An increasing number of surface‐associated proteins identified in Gram‐positive bacteria are characterized by intramolecular cross‐links in structurally conserved thioester, isopeptide, and ester domains (TIE proteins). TEDs are predicted at the distal end of a large number of surface proteins from Gram‐positive bacteria, and the name TIE (thioester, isopeptide, ester) proteins have been introduced for this family. Internal thioester bonds, formed between Cys and Gln side‐chains and first identified in the second thioester domain (TED) of the Streptococcus pyogenes minor pilin Cpa,3 play a negligible role in protein stability, but are suggested to mediate covalent bacterial adhesion. Structures of Bacillus anthracis, vancomycin‐resistant Staphylococcus aureus, and vancomycin‐resistant Enterococcus faecium TEDs show a head domain with Class I topology extended by a β‐sandwich; the latter contributes the thioester bond‐forming Gln via a β‐hairpin insertion into the head domain.

The B. anthracis BaTIE and the 86 kDa E. faecium EfmTIE86 proteins are predicted to comprise a Class II TED as well as three and five CnaB‐type isopeptide domains (IPDs), respectively. In addition to a TED and four IPDs, the S. aureus SaTIE protein is predicted to also contain two ester domains [Fig. 1(A)]. SaTIE is the only TIE protein so far identified in S. aureus. SaTIE‐TED (Gln254‐Gly502) and EfmTIE86‐TED (Asp39‐Ala314) were determined by ESI‐MS to be 17 Da lighter than predicted (suggesting the presence of a thioester bond), and readily yielded high‐quality crystals. SaTIE‐TED and EfmTIE86‐TED crystal structures were determined using Se‐SAD phasing and standard refinement procedures. Continuous electron density between Cys and Gln side‐chains either previously shown or predicted to form thioesters (SaTIE‐TED: Cys296 + Gln467,5 EfmTIE86‐TED: Cys88 + Gln292) confirmed the presence of these bonds. Despite pairwise identities of 18–23%, all three Class II TEDs in this study display very similar tertiary structures. In Class II TEDs, this loop is extended by approximately 15 residues, and covers the cleft between the β‐barrel and α‐helical subdomains. The specificity loop also contributes to forming a pore over 8 Å deep, the second restriction on access to the thioester bond [Fig. 5(C)]. The depth of this pore is longer than, for example, a Lys side‐chain (7 Å), strongly suggesting that in order for the thioester to interact with its cognate receptor, the surrounding tertiary structure must undergo a conformational change.

> GAMAQQKLDVKWIDKGINWIVYSAKDRENFTMDRWAKFYVNGEIAFCIEPNKEAAIGAVHTGANLDTLFKDQALRNKLTMISHFGYIANKDQSDEQYIATQMLIWELLGAKYHTIYNGLNYEARKADILKSVKEAEQRASFHKQKKPIKVGEKGVFVDTNNTLSNVKGIRTPSGVNAKIEGNKLIVTADKNAPDNATIHLDRITIVGTPLVYTSGNAQKVGVLKPFDPLDSWLTLQVIKNGNVKIIKEDTETG> MSNLSGTDKSVILLMTIGEDRAAEVFKHLSTREVQALSTAMANVRQISNKQLTDVLSEFEQEAE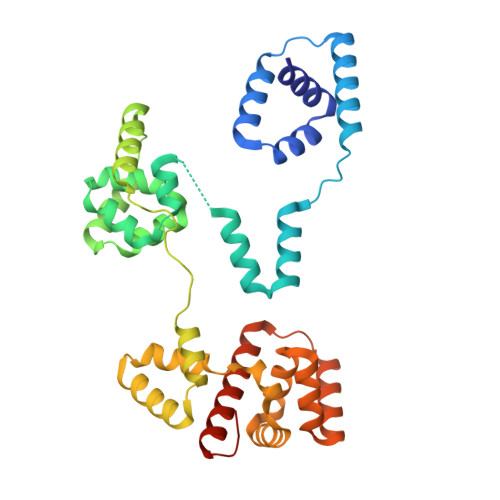QFAALNINANEYLRSVLVKALGEERASSLLEDILETRDTTSGIETLNFMEPQSAADLIRDEHPQIIATILVHLKRSQAADILALFDERLRHDVMLRIATFGGVQPAALAELTEVLNGLLDGQNLKRSKMGGVRTAAEIINLMKTQQEEAVITAVREFDGELAQKIIDEMFLFENLVDVDDRSIQRLLQEVDSESLLIALKGAEPPLREKFLRNMSQRAADILRDDLANRGPVRLSQVENEQKAILLIVRRLAETGEMVIGSGEDTYV>MLGSILPFNEETADRVSAYCEKNSHGIPDALVEHWEWTRTRFPDADKMSSRLQGSWMIFTARDRKPKRILEIGCYSGYSALAWYEGTRDTKAEIVTLEYSPKMIAASREAFKKYGVGDRVKLIEGPAENTLKTLEGEFDLIFVDANKDGYAGYVKTILDQGLLSANGIILCDNVFARGLTIGPDCAPWLNDHVRPYWNGCGQALDKFSAGLMEDPRIDVLLL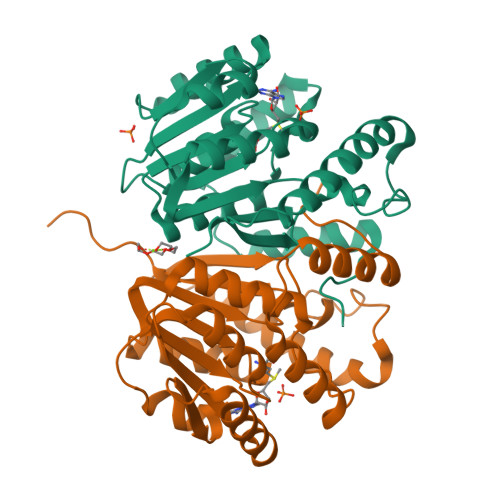PVFDGVTQIRWKDGAQRA[2x]>[2x]AGGHGDVGMHVKEKEKNKDENKRKDEERNKTQEEHLKEIMKHIVKIEVKG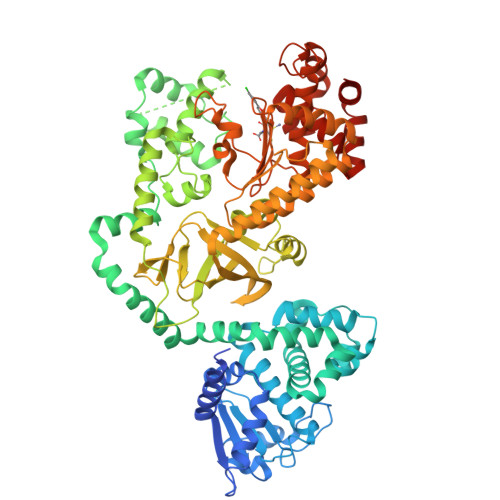EEAVKKEAAEKLLEKVPSDVLEMYKAIGGKIYIVDGDITKHISLEALSEDKKKIKDIYGKDALLHEHYVYAKEGYEPVLVIQSSEDYVENTEKALNVYYEIGKILSRDILSKINQPYQKFLDVLNTIKNASDSDGQDLLFTNQLKEHPTDFSVEFLEQNSNEVQEVFAKAFAYYIEPQHRDVLQLYAPEAFNYMDKFNEQEINLSLEELKDQRMLSRYEKWEKIKQHYQHWSDSLSEEGRGLLKKLQIPIEPKKDDIIHSLSQEEKELLKRIQIDSSDFLSTEEKEFLKKLQIDIRDSLSEEEKELLNRIQVDSSNPLSEKEKEFLKKLKLDIQPYDINQRLQDTGGLIDSPSINLDVRKQYKRDIQNIDALLHQSIGSTLYNKIYLYENMNINNLTATLGADLVDSTDNTKINRGIFNEFKKNFKYSISSNYMIVDINERPALDNERLKWRIQLSPDTRAGYLENGKLILQRNIGLEIKDVQIIKQSEKEYIRIDAKVVPKSKIDTKIQEAQLNINQEWNKALGLPKYTKLITFNVHNRYASNIVESAYLILNEWKNNIQSDLIKKVTNYLVDGNGRFVFTDITLPNIAEQYTHQDEIYEQVHSKGLYVPESRSILLHGPSKGVELRNDSEGFIHEFGHAVDDYAGYLLDKNQSDLVTNSKKFIDIFKEEGSNLTSYGRTNEAEFFAEAFRLMHSTDHAERLKVQKNAPKTFQFINDQIKFIINS>[3x]MWKRSEQMKIKSGKCNMAAAMETEQLGVEIFETADCEENIESQDRPKLEPFYVERYSWSQLKKLLADTRKYHGYMMAKAPHDFMFVKRNDPDGPHSDRIYYLAMSGENRENTLFYSEIPKTINRAAVLMLSWKPLLDLFQAT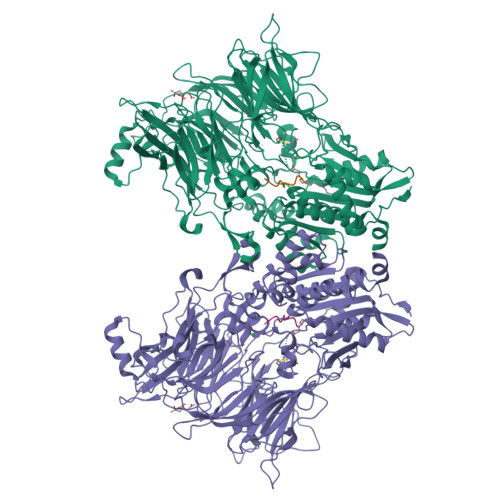LDYGMYSREEELLRERKRIGTVGIASYDYHQGSGTFLFQAGSGIYHVKDGGPQGFTQQPLRPNLVETSCPNIRMDPKLCPADPDWIAFIHSNDIWISNIVTREERRLTYVHNELANMEEDARSAGVATFVLQEEFDRYSGYWWCPKAETTPSGGKILRILYEENDESEVEIIHVTSPMLETRRADSFRYPKTGTANPKVTFKMSEIMIDAEGRIIDVIDKELIQPFEILFEGVEYIARAGWTPEGKYAWSILLDRSQTRLQIVLISPELFIPVEDDVMERQRLIESVPDSVTPLIIYEETTDIWINIHDIFHVFPQSHEEEIEFIFASECKTGFRHLYKITSILKESKYKRSSGGLPAPSDFKCPIKEEIAITSGEWEVLGRHGSNIQVDEVRRLVYFEGTKDSPLEHHLYVVSYVNPGEVTRLTDRGYSHSCCISQHCDFFISKYSNQKNPHCVSLYKLSSPEDDPTCKTKEFWATILDSAGPLPDYTPPEIFSFESTTGFTLYGMLYKPHDLQPGKKYPTVLFIYGGPQVQLVNNRFKGVKYFRLNTLASLGYVVVVIDNRGSCHRGLKFEGAFKYKMGQIEIDDQVEGLQYLASRYDFIDLDRVGIHGWSYGGYLSLMALMQRSDIFRVAIAGAPVTLWIFYDTGYTERYMGHPDQNEQGYYLGSVAMQAEKFPSEPNRLLLLHGFLDENVHFAHTSILLSFLVRAGKPYDLQIYPQERHSIRVPESGEHYELHLLHYLQENLGSRIAALKVI;>SLRFLYEG[3x]> MASMTGGQQMGRGSHHHHHHENLYFQGSDKGKLSLQDVAELIRARACQRVVVMVGAGISTPSGIPDFRSPGSGLYSNLQQYDLPYPEAIFELPFFFHNPKPFFTLAKELYPGNYKPNVTHYFLRLLHDKGLLLRLYTQNIDGLERVSGIPASKLVEAHGTFASATCTVCQRPFPGEDIRADVMADRVPRC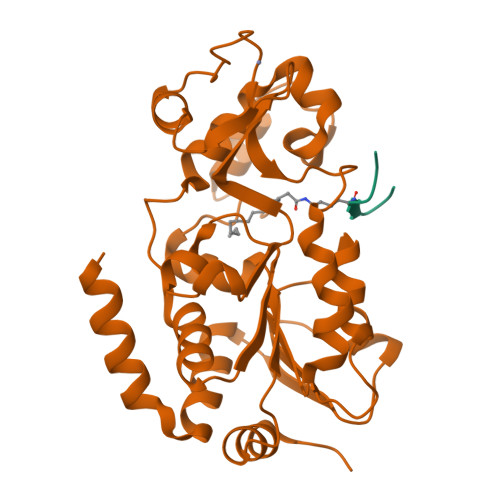PVCTGVVKPDIVFFGEPLPQRFLLHVVDFPMADLLLILGTSLEVEPFASLTEAVRSSVPRLLINRDLVGPLAWHPRSRDVAQLGDVVHGVESLVELLGWTEEMRDLVQRETGKLDGPDK;> QTARXSTGGW> MDRALPFIGDGLKPVQRRIVYAMSELGLNASAKFKKSARTV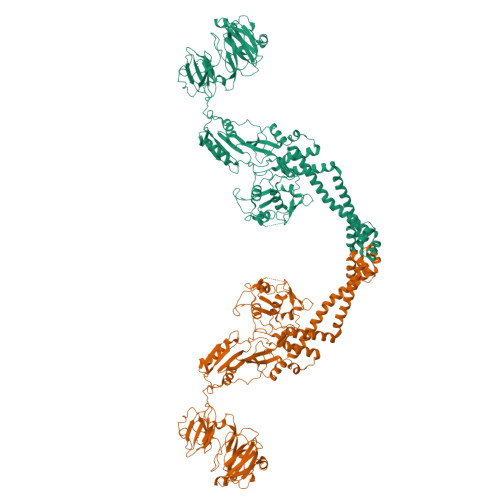GDVLGKYHPHGDSACYEAMVLMAQPFSYRYPLVDGQGNWGAPDDPKSFAAMRYTESRLSKYSELLLSELGQGTADWVPNFDGTLQEPKMLPARLPNILLNGTTGIAVGMATDIPPHNLREVAQAAIALIDQPKTTLDQLLDIVQGPDYPTEAEIITSRAEIRKIYENGRGSVRMRAVWKKEDGAVVISALPHQVSGARVLEQIAAQMRNKKLPMVDDLRDESDHENPTRLVIVPRSNRVDMDQVMNHLFATTDLEKSYRINLNMIGLDGRPAVKNLLEILSEWLVFRRDTVRRRLNYRLEKVLKRLHILEGLLVAFLNIDEVIEIIRNEDEPKPALMSRFGLTETQAEAILELKLRHLAKLEEMKIRGEQSELEKERDQLQGILASERKMNNLLKKELQADAQAYGDDRRSPLQEREEAKAMSEHDMLPSEPVTIVLSQMGWVRSAKGHDIDAPGLNYKAGDSFKAAVKGKSNQPVVFVDSTGRSYAIDPITLPSARGQGEPLTGKLTLPPGATVDHMLMESDDQKLLMASDAGYGFVCTFNDLVARNRAGKALITLPENAHVMPPVVIEDASDMLLAITQAGRMLMFPVSDLPQLSKGKGNKIINIPSAEAARGEDGLAQLYVLPPQSTLTIHVGKRKIKLRPEELQKVTGERGRRGTLMRGLQRIDRVEIDSP> PPPPM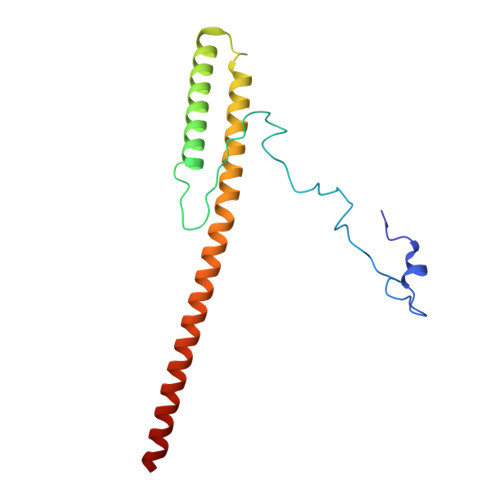QYIKEYTDENIQEGLAPKPPPPIKDSYMMFGNQFQCDDLIIRPLESQGIERLHPMQFDHKKELRKLNMSILINFLDLLDILIRSPGSIKREEKLEDLKLLFVHVHHLINEYRPHQARETLRVMMEVQKRQRLETAERFQKHLERVIEMIQNC>[6x]SNAMNDWASLGIGSIGEAVFSKLLKVVIDEAKKFKAFKPLSK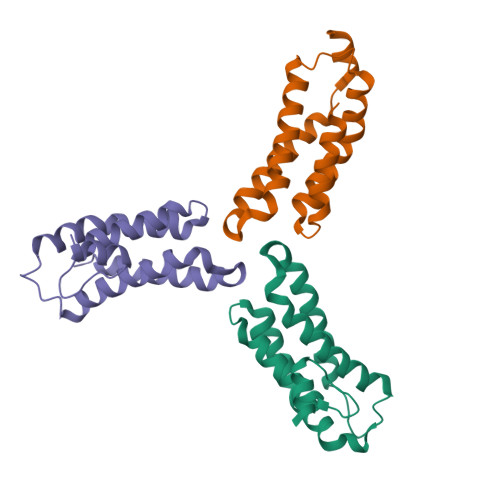DLVSTMEILFPLTQKIDSMQKELDFGVKELKELRDTIERADVAVRKFPRVKWYEESEYTEEIEEINEDMLEFCQIDLQLLQHRNQWSHPQFEK2-[(1S)-1-[4-[2-(4-chloranylphenoxy)ethanoyl]piperazin-1-yl]ethyl]-3-(2-ethoxyphenyl)quinazolin-4-one | C30 H31 Cl N4 O4 | 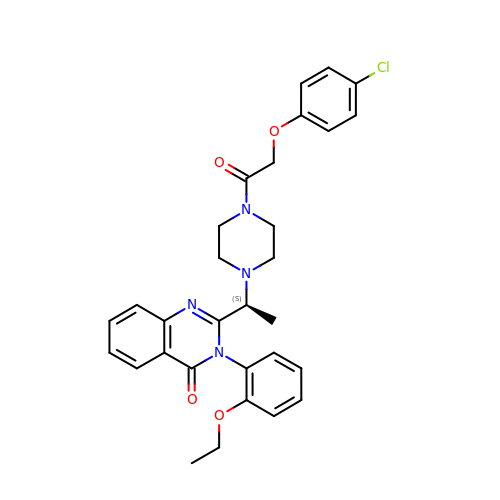BKQFRNYHFIQEKN-NRFANRHFSA-N>MLAKRIIACLDVKDGRVVKGTNFENLRDSGDPVELGKFYSEIGIDELVFLDITASVEKRKTMLELVEKVAEQIDIPFTVGGGIHDFETASELILRGADKVSINTAAVENPSLITQIAQTFGSQAVVVAIDAKRVDGEFMVFTYSGKKNTGILLRDW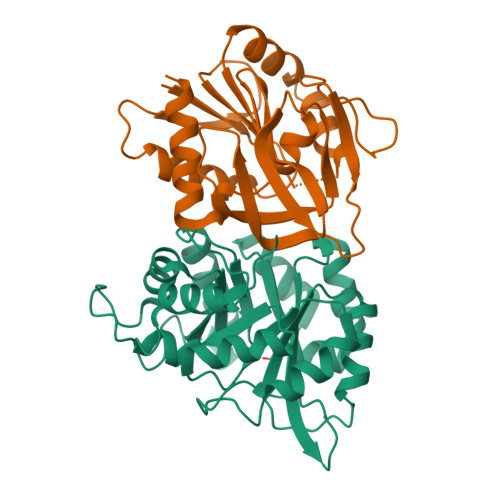VVEVEKRGAGEILLTSIDRDGTKSGYDTEMIRFVRPLTTLPIIASGGAGKMEHFLEAFLAGADAALAASVFHFREIDVRELKEYLKKHGVNVRLEGL[3x];>MRIGIISVGPGNIMNLYRGVKRASENFEDVSIELVESPRNDLYDLLFIPGVGHFGEGMRRLRENDLIDFVRKHVEDERYVVGVCLGMQLLFEESEEAPGVKGLSLIEGNVVKLRSRRLPHMGWNEVIFKDTFPNGYYAFVHTYRAVCEEEHVLGTTEYDGEIFPSAVRKGRILGFQFHPEASSKIGRKLLEKVIECSLSRR[3x]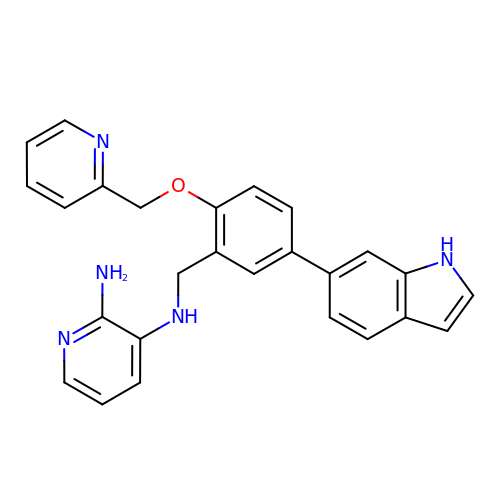N~3~-[5-(1H-INDOL-6-YL)-2-(PYRIDIN-2-YLMETHOXY)BENZYL]PYRIDINE-2,3-DIAMINE | C26 H23 N5 O | KMBPJSHPAXOXBT-UHFFFAOYSA-N> MMINTQEDKLVSAHDAEEFHRFFVGHDSDLQQEVTTLLTREAHLLDIQAYKAWLEHFVAPEIKYQVISRELRSTSERRYQLNDAVNLYNENYQQLKVRVEHQMDPQNWANNPKIRFTRFVTNVTAAKDKSAPEILHVRSNLILHRARRENQVDVFYATREDK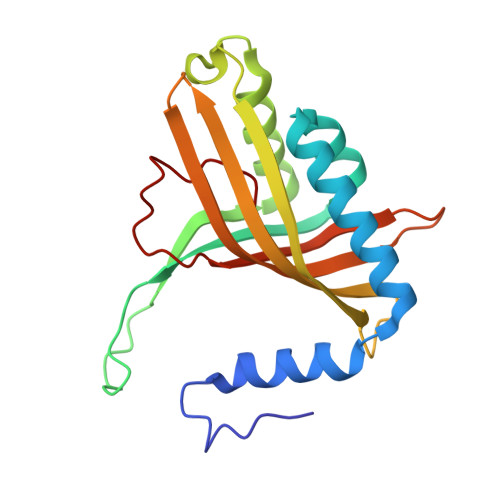WKRIEGGGIKLVERFVDYPERIPQTHNLLVFL O-phosphono-N-(9-sulfanylnonanoyl)-L-threonine | C13 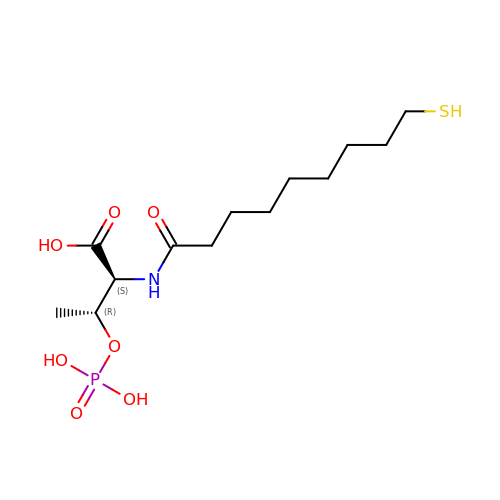H26 N O7 P S | WUTPSGIFCCYDED-PWSUYJOCSA-N> DPGTHIVLWTGDQELELQRLFEEFRDSDDVLGHIMKNITAKRSRARIVDKLLALGL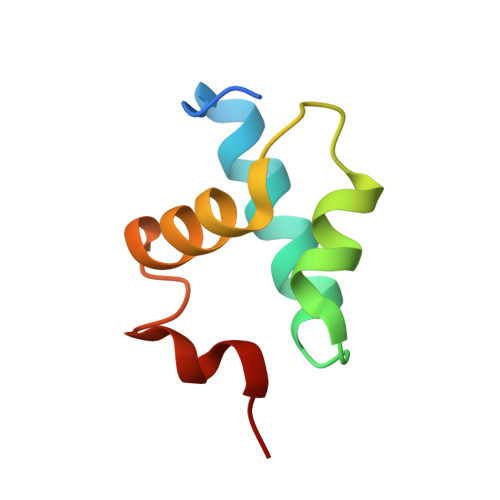VAERRELYKKR>MGSSHHHHHHSSENLYFQGHMADQDHAQLLHVLGIENLRRGADGNTDSPFAANTDEAKANTALDSLPPLLTSVSGQAIASATDWEANRPALLNTFSQEIYGYVPGGAPELHWKAGSTTPIDDSGTSAIRQHFTSTLVHPENAALNLSLNFTLVLPKSNKPVPVVVVMSFDPGIWERFRDRMPAERYAQIQADNARWREQVVNAGWGYAEIIPTEFQADSGDGLSQGIIGFVNNGKPRNPTDWGALRAWAWSASQVLTYLQTDSRVAADRISVHGHSRFGKAALVAMAFDNRFAAGFISSSGEGGAKLWRRNFGEQVGNLAGAGEYHWMAGNFVKYAGPKKVNDIPVDAHQLLALCAPRPVLVSVGSQGESWVDPKGMLLAAYHATPAYALFGEQGVTQNELPAVGNGLLAGKLAFRQHEGGHTPAPNWETFITFATRQWA[3x]

The aim of the present study was to investigate structure-function relationships of TtCE15A, a novel CE15 enzyme from the Gram-negative bacterium Teredinibacter turnerae. T. turnerae has been isolated from the gills of a wood-boring shipworm, a mollusk that digests lignocellulose in marine environments. TtCE15A has an α/β-hydrolase fold similar to previously determined CE15 structures, consisting of a three-layer sandwich with a solvent-exposed cleft comprising the active site with its catalytic triad.

Three TtCE15A molecules were found in the asymmetric unit, with a Cα root mean square deviation below 0.2 Å (all atoms <1 Å), indicating a high degree of similarity between the protein chains. Like the previously determined bacterial structures, TtCE15A has three inserted regions relative to the fungal CE15 structures (Reg1, residues 122–134; Reg2, 175–200; Reg3, 399–415). Although being shorter in sequence (26 versus 40–45 residues), Reg2 of TtCE15A forms a much longer helix compared with the Regs2 of OtCE15A, SuCE15C, and MZ0003. The longer Reg2 helix present in TtCE15A builds up a larger ridge around the previously proposed lignin-binding region and thus presents a deeper substrate-binding groove compared with previously solved structures. On the ridge built up by Reg2, multiple hydrophobic residues are found on the side facing the active site (Phe-174, Ile-178, Trp-179, Phe-182, Met-186, and Ile-194), whereas the opposite face is more hydrophilic. At the N terminus, TtCE15A has an additional extension (RegN, residues 27–55) consisting of ∼30 residues neighboring the previously proposed xylan-binding region. RegN forms a further deepening of the active site pocket opposite Reg2, a feature not present in any previously determined CE15 structure. The serine and histidine residues of the catalytic triad found in all previously solved structures (fungal and bacterial) are conserved in TtCE15A (Ser-281 and His-427). However, the proposed canonical glutamate of the catalytic triad is absent (similar to MZ0003), and this position is occupied by a serine residue (Ser-304). In TtCE15A, a glutamate, Glu-374, is found in an equivalent position, which would likely fulfill the same role.> SDVCPLTLGIETVGGVMTKLIPRNTVVPTKKSQIFSVGGTVTIKVYEGERPLTKDNHLLGTFDLTGIPPAPRGVPQIEVTFEIDVNGILRVTAEDKGTGNKNKITITNDQNRLTPEEIERMVNDAEKFAEEDKKLKERIDTRNELESYAYSLKNQIGDKEKLGGKLSSEDKETMEKAVEEKIEWLESHQDADIEDFKAKKKELEEIVQPIISKLYGSENLYFQGSNRLLLT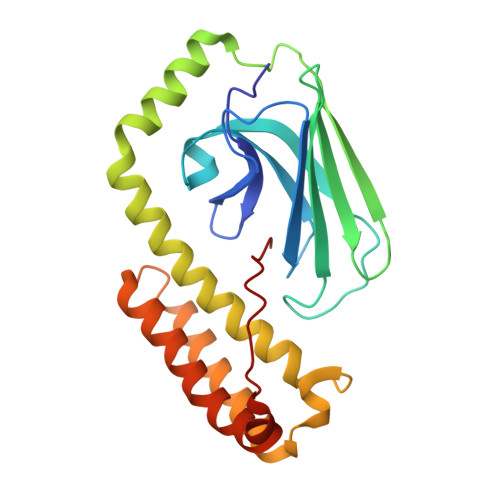G> MNTINIAKNDFSDIELAAIPFNTLADHYGERLAREQLALEHE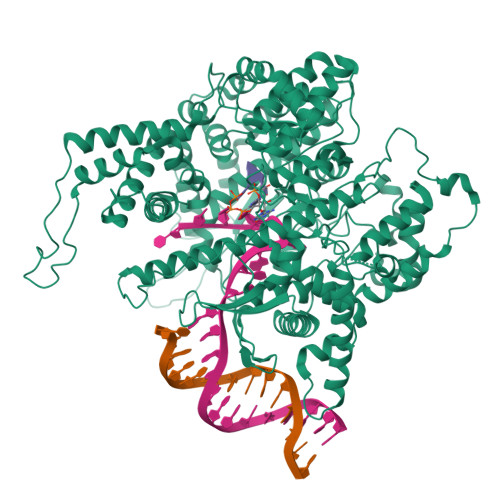SYEMGEARFRKMFERQLKAGEVADNAAAKPLITTLLPKMIARINDWFEEVKAKRGKRPTAFQFLQEIKPEAVAYITIKTTLACLTSADNTTVQAVASAIGRAIEDEARFGRIRDLEAKHFKKNVEEQLNKRVGHVYKKAFMQVVEADMLSKGLLGGEAWSSWHKEDSIHVGVRCIEMLIESTGMVSLHRQNAGVVGQDSETIELAPEYAEAIATRAGALAGISPMFQPCVVPPKPWTGITGGGYWANGRRPLALVRTHSKKALMRYEDVYMPEVYKAINIAQNTAWKINKKVLAVANVITKWKHCPVEDIPAIEREELPMKPEDIDMNPEALTAWKRAAAAVYRKDKARKSRRISLEFMLEQANKFANHKAIWFPYNMDWRGRVYAVSMFNPQGNDMTKGLLTLAKGKPIGKEGYYWLKIHGANCAGVDKVPFPERIKFIEENHENIMACAKSPLENTWWAEQDSPFCFLAFCFEYAGVQHHGLSYNCSLPLAFDGSCSGIQHFSAMLRDEVGGRAVNLLPSETVQDIYGIVAKKVNEILQADAINGTDNEVVTVTDENTGEISEKVKLGTKALAGQWLAYGVTRSVTKRSVMTLAYGSKEFGFRQQVLEDTIQPAIDSGKGLMFTQPNQAAGYMAKLIWESVSVTVVAAVEAMNWLKSAAKLLAAEVKDKKTGEILRKRCAVHWVTPDGFPVWQEYKKPIQTRLNLMFLGQFRLQPTINTNKDSEIDAHKQESGIAPNFVHSQDGSHLRKTVVWAHEKYGIESFALIHDSFGTIPADAANLFKAVRETMVDTYESCDVLADFYDQFADQLHESQLDKMPALPAKGNLNLRDILESDFAFA> MSLKPVMIIQFSASEGPGHFGDFLAGEHIPFQVLRMDRSDPLPAEIRDCSGLAMMGGPMSANDDLPWMPTLLALIRDAVAQRVPVIGHCLGGQLLAKAMGGEVTDSPHA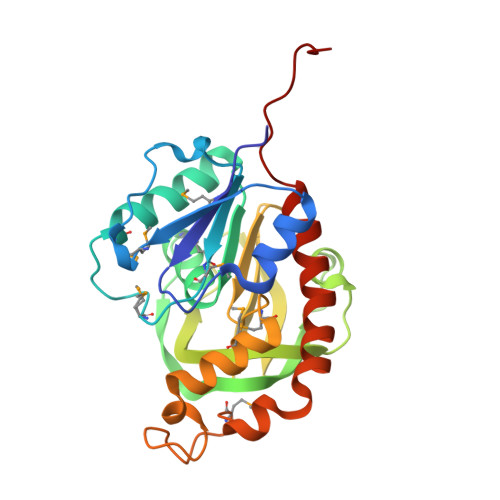EIGWVRAWPQHVPQALEWLGTWDELELFEWHYQTFSIPPGAVHILRSEHCANQAYVLDDLHIGFQCHIEMQAHMVREWCSISPEELKGGAEADPAQPMVQSAVEILRDLDVRIATLNRWAEHVYARWIKGLQREGHHHHHH> LESHMTPKDDEFYQQWQLKYPK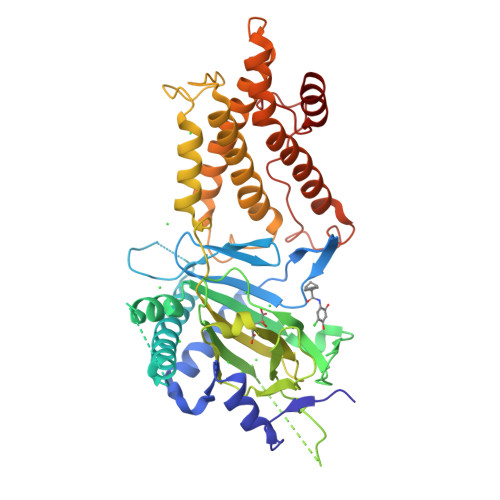LILREASSVSEELHKEVQEAFLTLHKHGCLFRDLVRIQGKDLLTPVSRILIGNPGCTYKYLNTRLFTVPWPVKGSNIKHTEAEIAAACETFLKLNDYLQIETIQALEELAAKEKANEDAVPLCMSADFPRVGMGSSYNGDVEVDIKSRAAYNVTLLNFMDPQKMPYLKEEPYFGMGKMAVSWHHDENLVDRSAVAVYSYSCEGPEEESEDDSHLEGRDPDIWHVGFKISWDIETPGLAIPLHQGDCYFMLDDLNATHQHCVLAGSQPRFSSTHRVAECSTGTLDYILQRCQLALQNVCDDVDNDDVSLKSFEPAVLKQGEEIHNEVEFEWLRQFWFQGNRYRKCTDWWCQPMAQLEALWKKMEGVTNAVLHEVKREGLPVEQRNEILTAILASLTARQNLRREWHARCQSRIARTLPADQKPECRPYWEKDDASMPLPFDLTDIVSELRGQLLEAKP> MGSSLRPLYMDVQATTPLDPRVLDAMLPYLINYYGNPHSRTHAYGWESEAAMERARQQVASLIGADPREIIFTSGATESNNIAIKGVARFYRSRKKHLITTQTEHKCVLDSCRSLEAEGFQVTYLPVQKSGIIDLKELEAAIQPDTSLVSVMTVNNEIGVKQPIAEI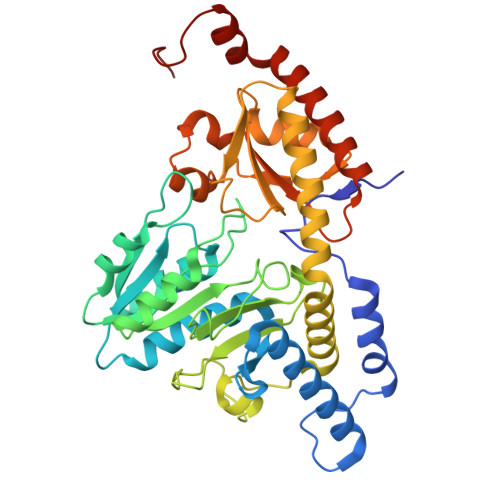GRICSSRKVYFHTDAAQAVGKIPLDVNDMKIDLMSISGHKIYGPKGVGAIYIRRRPRVRVEALQSGGGQERGMRSGTVPTPLVVGLGAACEVAQQEMEYDHKRISKLSERLIQNIMKSLPDVVMNGDPKHHYPGCINLSFAYVEGESLLMALKDVALSSGSACTSASLEPSYVLRAIGTDEDLAHSSIRFGIGRFTTEEEVDYTVEKCIQHVKRLREMSPLWEMVQDGIDLKSIKWTQH>[2x]MMANRMILNETAWFGRGAVGALTDEVKRRGYQKALIVTDKTLVQCGVVAKVTDKMDAAGLAWAIYDGVVPNPTITVVKEGLGVFQNSGADYLIAIGGGSPQDTCKAIGIISNNPEFADVRSLEGLSPTNKPSVPILAIPTTAGTAAEVTIGYVITDEEKRRKFVCVDPHDIPQVAFIDADMMDGMPPALKAATGVDALTHAIEGYITRGAWALTDALHIKAIEIIAGALRGSVAGDKDAGEEMALGQYVAGMGFSNVGVGLVHGMAHPLGAFYNTPHGVANAILLPHVMRYNADFTGEKYRDIARVMGVKVEGMGLEEARNAAVEAVFALNRDVGIPPHLRDVGVRKEDIPALAQAALDDVCTGGNPREATLEDIVELYHTAWTSHHHHH

Here it is shown which structural adaptations were introduced by directed evolution experiments that changed the catalytic properties of the Escherichia coli (E. coli) (S)-lactaldehyde reductase [EC 1.1.1.77]. This enzyme, referred to as FucO, is also known as an Fe2+, NAD+-dependent group-III alcohol de­hydrogenase and is involved in the catabolism of rare sugars in E. coli.

The isolated DA1472 variant is a double point mutation variant, N151G and L259V. The mode of binding of NADH in the active site, including the nicotinamide moiety, is well defined by the electron density map, being the same in both structures. The structures of the protein regions with the mutated residues are well defined by the electron density maps and the conformations of these regions are the same as in the wild-type. The comparison of the structures of the active sites of the wild-type and the DA1472 variant shows that the shorter side chains of the L259V (valine instead of leucine) and N151G (glycine instead of asparagine) amino acid substitutions provide more space in the region where the substrate binds. The structural data show that the two amino acid changes (N151G and L259V) do not cause any change of main-chain conformation, but do provide more space in the substrate-binding groove. Also, the geometry of the catalytic site is not affected and the enzymological data suggest that the reaction mechanism of the DA1472 variant is also the same. The results illustrate a dramatic shift in substrate scope. The preference of the wild-type enzyme for short-chain aliphatic 2-hy­droxy­aldehydes has been shifted to favor aryl-substituted, non-hydroxy­lated aldehydes. k cat/K M for phenyl­acetaldehyde (compound 3) has increased approximately 9000-fold whereas the activity with the native (S)-lactaldehyde (compound 2) has decreased approximately 80-fold.>MGGSHHHHHHENLYFQGMSKSKVDNQFYSVEVADSTFTVLKRYQQLKPIGSGAQGIVCAAFDTVLGINVAVKKLSRPFQNQTHAKRAYRELVLLKCVNHKNIISLLNVFTPQKTLEEFQDVYLVMELMDANLCQVIHMELDHERMSYLLYQMLCGIKHLHSAGIIHRDLKPSNIVVKSDCTLKILDFGLARTACTNFMMTPYVVTRYYRAPEVILGMGYAANVDIWSVGCIMGELVKGCVIFQGTDHIDQWNKVIEQLGTPSAEFMAALQPTVRNYVENRPKYPGIKFEELFPDWIFPSESERDKIKTSQARDLLSKMLVIDPDKRISVDEALR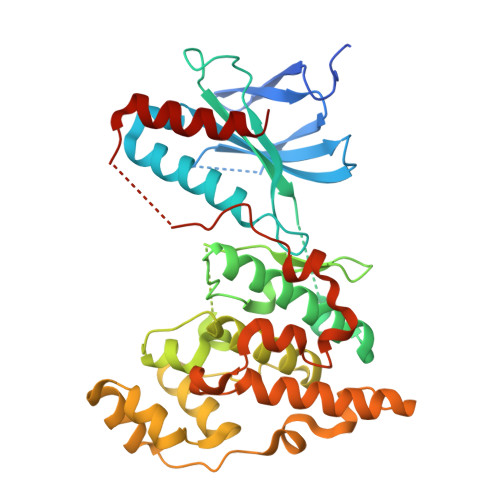HPYITVWYDPAEAEAPPPQIYDAQLEEREHAIEEWKELIYKEVMDWE[2x]> NLVQFSYLIQCANHGKRPTWHYMDYGCYCGAGGSGTP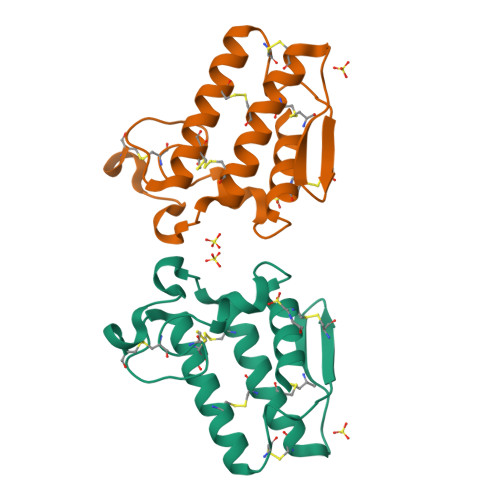VDELDRCCKIHDDCYDEAGKKGCFPKMSAYDYYCGENGPYCRNIKKKCLRFVCDCDVEAAFCFAKAPYNNANWNIDTKKRCQ>[2x]GPLGSMFSVESLERAELCESLLTWIQTFNVDAPCQTVEDLTNGVVMAQVLQKIDPAYFDENWLNRIKTEVGDNWRLKISNLKKILKGILDYNHEILG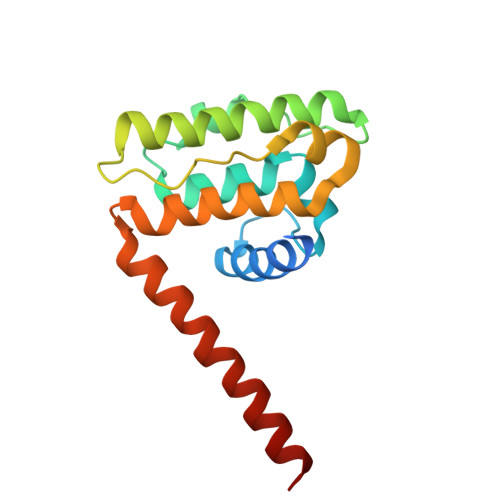QQINDFTLPDVNLIGEHSDAAELGRMLQLILGCAVNCEQKQEYIQAIMMMEESVQHVVMTAIQELMSK> GELVRTDSPNFLCSVLPTHWRCNKTLPIAFKVVAKGDVPDGTLVTVMAGNDENYSAELRNATAAMKNQVARFNDLRFVGRSGRGKSFTLTITVFTNPPQVATYHRA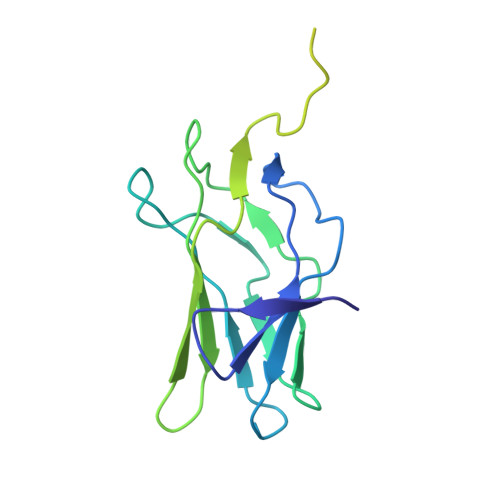IAITVDGPREPRRHRQKLDDQTKPGSLSFSERLSELEQLRRTAMRVSPHHPAPTPNPRASLNHSTAFNPQPQSQMQDARQIQPSPPWSYDQSYQYLGS> DRHHHHHHKLPEEQKVLVVSFDGFRWDYLYKVPTPHFHYIMKNGVHVNQVTNVFITKAYPNHYTLVTGLFAENHGIVANDMFDPILNKSFSLEHMDIYDSKFWEEATPIWITNQRAGHASGAAMWPGADVKIHDSFPTYYLPYNESVSFEDRVAKIIEWFTAKDPINLGFLYWEEPDDTGHDVGPDSPLMGSVISDVDHKLGYLIKMLKRAKLWNNVNLIVTSDHGMTQCSKQRV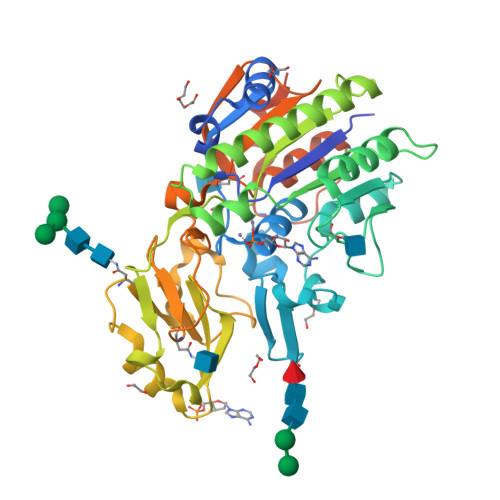IELDRYLDKEHYTLIDHSPVAAILPKEGKFDEVYDALAGAHPNLTVYKKEEIPERWHYKHNDRVQPIVAVADEGWYILQNKSDDFLLGNHGYDNALAEMHPIFLAHGPAFRKNFTKEAMNSTDLYSLLCHLLNLTALPHNGSFWNVQDLLSSATPKPIPYTQSTTLLLGSDKPGEDEQEES>MMGSSHHHHHHHHHSSGENLYFQGGSMIEVTEVSIAELRDALESGRTTAVELVQAYLARIDAYDAPGTPTALNAVVVRNPDALAEAQASDARRARGEPLGPLDGIPYTAKDSYLVKGLTAASGSPAFKDLVAQRDAFTVERLRAAGAICLGKTNMPPMANGGMQRGVYGRAESPYNAAYLTAPFASGSSNGAGTATAASFAAFGLAEETWSSGRGPASNNGLCAYTPSRGVISVRGNWPLTPTMDVVVPYARSMADLLEILDVVVADDPDTRGDLWRMQPWVPIPKASEVRPASYPALAAGAEALAGKRFGVPRMFINADPDAGTSESPGIGGPTGQRIHTRPSVIALWEQARKALEAAGAEVIEVDFPLVSNCEGDRPGAPTVFNRGLVSKEFLHDELWELSAWGFDDFLRANGDPKLNRLA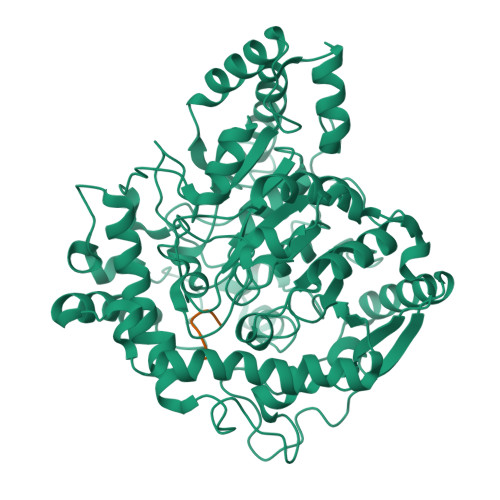DVDGPQIFPHDPGTLPNREGDLAAGMDEYVRMAERGIKPWDRIATLPDGLRGLEETRRIDLEEWMRRLRLDAVLFPTVADVGPADADVNPASADIAWSNGVWVANGNLAIRHLGVPTVTVPMGVMADIGMPVGLTFAGRAYDDSALLRFAAAFESTGSRRIVPPRTPPLASK[2x];> PPLASK> GSHMNREMLYLNRSDIEQAGGNHSQVYVDALTEALTAHAHNDFVQPLKPYLRQDPENGHIADRIIAMPSHIGGEHAISGIKWIGSKHDNPSKRNMERASGVIILNDPETNYPIAVMEASLISSMRTAAVSVIAAKHLAKKGFKDLTIIGCGLIGDKQLQSMLEQFDHIERVFVYDQFSEACARFVDRWQQQRPEINFIATENAKEAVSNGEVVITCTVTDQPYIEYDWLQKGAFISNISIMDVHKEVF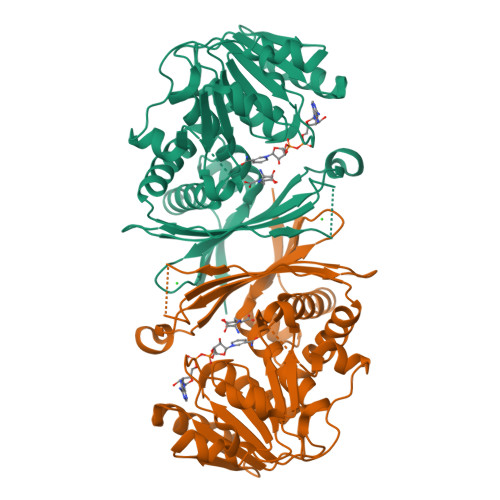IKADKVVVDDWSQCNREKKTINQLVLEGKFSKEALHAELGQLVTGDIPGREDDDEIILLNPMGMAIEDISSAYFIYQQAQQQNIGTTLNLY> MNIIAIMGPHGVFYKDEPIKELESALVAQGFQIIWPQNSVDLLKFIEHNPRICGVIFDWDEYSLDLCSDINQLNEYLPLYAFINTHSTMDVSVQDMRMALWFFEYALGQAEDIAIRMRQYTDEYLDNITPPFTKALFTYVKERKYTFCTPGHMGGTAYQKSPVGCLFYDFFGGNTLKADVSISVTELGSLLDHTGPHLEAEEYIARTFGAEQSYIVTNGTSTSNKIVGMYAAPSGSTLLIDRNCHKSLAHLLMMNDVVPVWLKPTRNALGILGGIPRREFTRDSIEEKVAATTQAQWPVHAVITNSTYDGLLYNTDWIKQTLDVPSIHFDSAWVPYTHFHPIYQGKSGMSGERVAGKVIFETQSTHKMLAALSQASLIHIKGEYDEEAFNEAFMMHTTTSPSYPIVASVETAAAMLRGNPGKRLINRSVERALHFRKEVQRLREESDGWFFDIWQPPQVDEAECWPVAPGEQWHGFNDADADHMFLDPVKVTILTPGMDEQGNMSEEGIPAALVAKFLDERGIVVEKTGPYNLLFLFSIGIDKTKAMGLLRGLTEFKRSYDLNLRIKNMLPDLYAEDPDFYRNMRIQDLAQGIHKLIRKHDLPGLMLRAFDTLPEMIMTPHQAWQRQIKGEVETIALEQLVGRVSANMILPYPPGVPLLMPGEMLTKESRTVLDFLLMLCSVG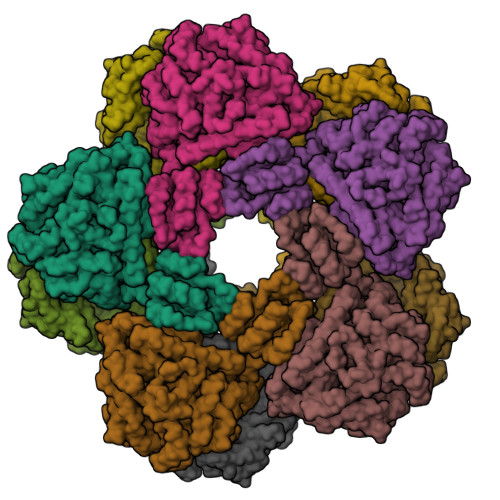QHYPGFETDIHGAKQDEDGVYRVRVLK> TNLYMLPK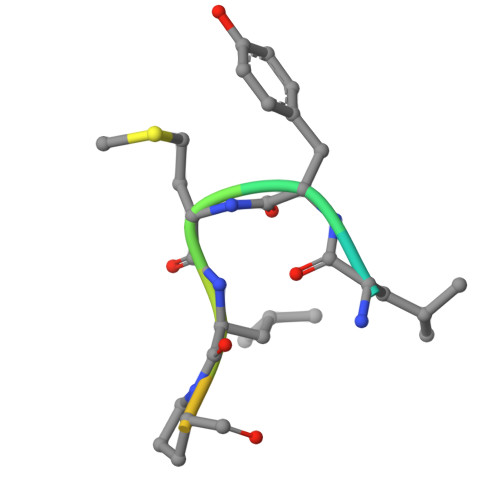WDIP>MSDKTKTNEGFSRRSFIGSAAVVTAGVAGLGAIDAASATQKTNRASTVKGGFDYDVVVVGGGFAGATAARECGLQGYRTLLLEARSRLGGRTFTSRFAGQEIEFGGAWVHWLQPHVWAEMQRYGLGVVEDPLTNLDKTLIMYNDGSVESISPDEFGKNIRIAFEKLCHDAWEVFPRPHEPMFTERARELDKSSVLDRIKTLGLSRLQQAQINSYMALYAGETTDKFGLPGVLKLFACGGWNYDAFMDTETHYRIQGGTIGLINAMLTDSGAEVRMSVPVTAVEQVNGGVKIKTD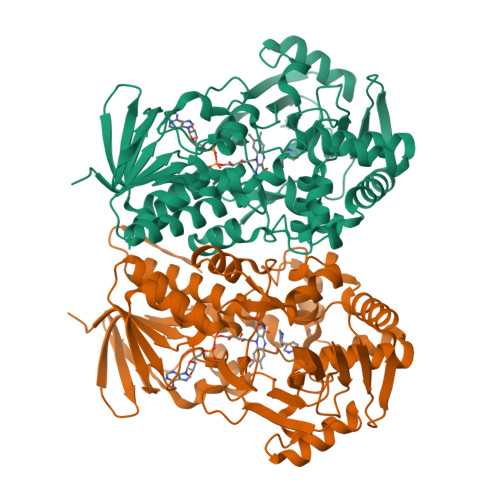DDEIITAGVVVMTVPLNTYKHIGFTPALSKGKQRFIKEGQLSKGAKLYVHVKQNLGRVFAFADEQQPLNWVQTHDYSDELGTILSITIARKETIDVNDRDAVTREVQKMFPGVEVLGTAAYDWTADPFSLGAWAAYGVGQLSRLKDLQAAEGRILFAGAETSNGWHANIDGAVESGLRAGREVKQLLSLEHHHHHH[4x]>SNAADPKTKGRGSGGNGSGRRLVIVESPTKARKLASYLGSGYIVESSRGHIRDLPRAASDVPAKYKSQPWARLGVNVDADFEPLYIISPEKRSTVSELRGLLKDVDELYLATDGDREGEAIAWHLLETLKPRIPVKRMVFHEITEPAIRAAAEHPRDLDIDLVDAQETRRILDRLYGYEVSPVLWKKVAPKLSAGRVQSVATRIIVARERDRMAFRSAAYWDILAKLDASVSDPDAAPPTFSARLTAVAGRRVATGRDFDSLGTLRKGDEVIVLDEGSATALAAGLDGTQLTVASAEEKPYARRPYPPFMTSTLQQEASRKLRFSAERTMSIAQRLYENGYITYMRTDSTTLSESAINAARTQARQLYGDEYVAPAPRQYTRKVKNAQEAHEAIRPAGETFATPDAVRRELDGPNIDDFRLYELIWQRTVASQMADARGMTLSLRITGMSGHQEVVFSATGRTLTFPGFLKAYVETVDELVGGEADDAERRLPHLTPGQRLDIVELTPDGHATNPPARYTEASLVKALEELGIGRPSTYSSIIKTIQDRGYVHKKGSALVPSWVAFAVTGLLEQHFGRLVDYDFTAAMEDELDEIAAGNERRTNWLNNFYFGGDHGVPDSVARSGGLKKLVGINLEGIDAREVNSIKLFDDTHGRPIYVRVGKNGPYLERLVAGDTGEPTPQRANLSDSITPD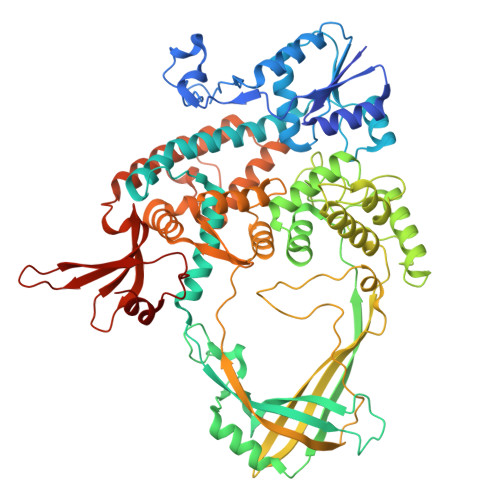ELTLQVAEELFAT[2x]>ACQDPTIFEERHLKYISQLGKGNFGSVELCRYDPLGDNTGALVAVKQLQHSGPDQQRDFQREIQILKALHSDFIVKYRGVSYGPGRQSLRLVMEYLPSGCLRDFLQRHRARLDAS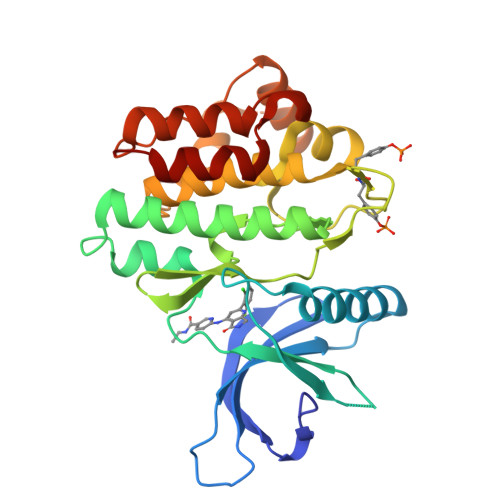RLLLYSSQICKGMEYLGSRRCVHRDLAARNILVESEAHVKIADFGLAKLLPLDKDYYVVREPGQSPIFWYAPESLSDNIFSRQSDVWSFGVVLYELFTYCDKSCSPSAEFLRMMGSERDVPALSRLLELLEEGQRLPAPPACPAEVHELMKLCWAPSPQDRPSFSALGPQLDMLWS[4x]> ESQPDPMPDDLHKSSEFTGTMGN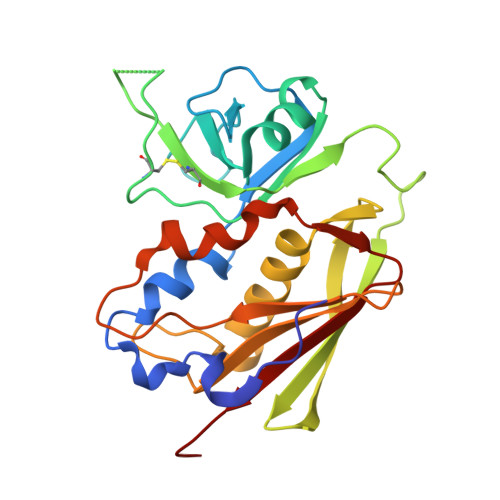MKYLYDDHYVSATKVKSVDKFLAHDLIYNISDKKLKNYDKVKTELLNEDLAKKYKDEVVDVYGSNYYVNCYFSSKDNKASTWHGKTCMYGGITKHEGNHFDNGNLQNVLVRVYENKRNTISFEVQTDKKSVTAQELDIKARNFLINKKNLYEFNSSPYETGYIKFIENNGNTFWYDMMPAPGDKFDQSKYLMMYNDNKTVDSKSVKIEVHLTTKNG>[2x]QARILEADARILQAYANILS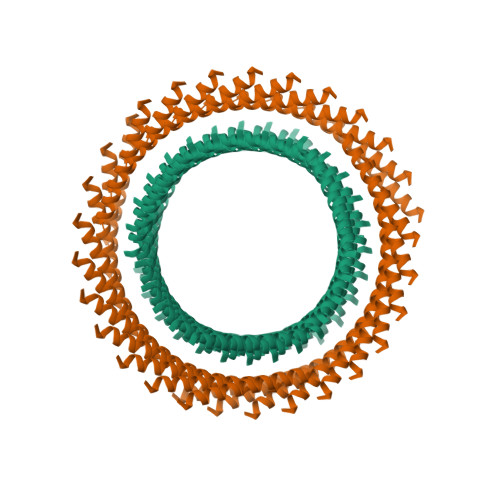AHAEILRAE> TGSYDPCTERYSTAYYNRRDVQMALHANVTGAMNYTWATCSDTINTHWHDAPRSMLPIYRELIAAGLRIWV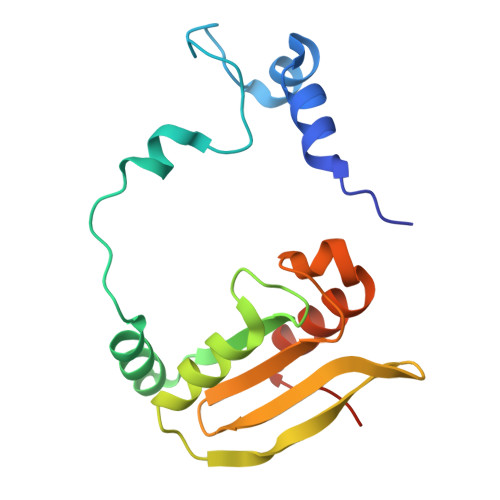FSGDTDAVVPLTATRYSIGALGLPTTTSWYPWYDDQEVGGWSQVYKGLTLVSVRGAGHEVPLHRPRQALVLFQYFLQGKPMPGQTKNAT> MSRQSISLRFPLLLLLLSPSPVFSADPGAPAPVNPCCYYPCQHQGICVRFGLDRYQCDCTRTGYSGPNCTIPEIWTWLRTTLRPSPSFIHFLLTHGRWLWDFVNATFIRDTLMRLVLTVRSNLIPSPPTYNIAHDYISWESFSNVSYYTRILPSVPRDCPTPMGTKGKKQLPDAEFLSRRFLLRRKFIPDPQGTNLMFAFFAQHFTHQFFKTSGKMGPGFTKALGHGVDLGHIYGDNLERQYQLRLFKDGKLKYQMLNGEVYPPSVEEAPVLMHYPRGIPPQSQMAVGQEVFGLLPGLMLYATIWLREHNRVCDLLKAEHPTWGDEQLFQTARLILIGETIKIVIEEYVQQLSGYFLQLKFDPELLFGAQFQYRNRIAMEFNQLYHWHPLMPDSFRVGPQDYSYEQFLFNTSMLVDYGVEALVDAFSRQPAGRIGGGRNIDHHILHVAVDVIKESRVLRLQPFNEYRKRFGMKPYTSFQELTGEKEMAAELEELYGDIDALEFYPGLLLEKCHPNSIFGESMIEMGAPFSLKGLLGNPICSPEYWKASTFGGEVGFNLVKTATLKKLVCLNTKTCPYVSFH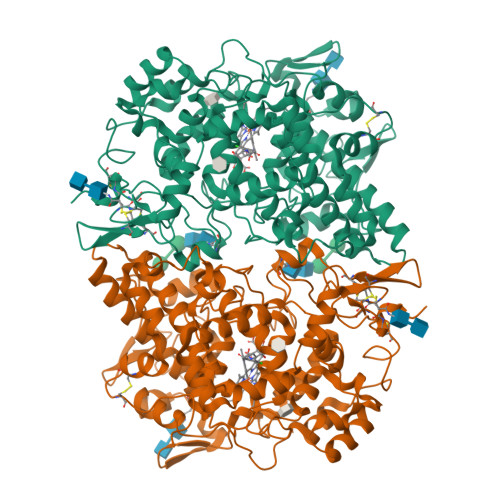VPDPRQEDRPGVERPPTEL> MKQGFARPTPERAPVVKPENIVLPTPLSVPPPEGKPWWLVVVGVLVVGLLVGMVGMTVASGSRLFLGAGAIFPIFMIGGVAMMMFGGRFGGQQQMSRPKLDAMRAQFMLMLDMLRETAQESADSMDANYRWFHPAPTTLAAAVGSSRMWERQPDGKDLNFGVVRVGVGMTRPEVTWGEPQNMPTDIELEPVTGKALQEFGRYQSVVYNLPKMVSLLVEPWYSLVGEREQVLGLTRAIICQLAFSHGPDHVQMIVVTSDPDRWDWVKWIPHFGDPRRRDAAGNARMVYTSVREFATEQAELFAGRGSFTPRHASSSAETPTPHHVIISDIEDPQWEYVISSEGVDGVTFFDLTGSPLWTGAPQRVLRFTDSAGVIETLPRDRDTWMVIDDNAWFFALADQMSEADAEQFAHQMAHWRLAEAYEEIGQRVVQLGARDILSYYGIDDAGEIDFNT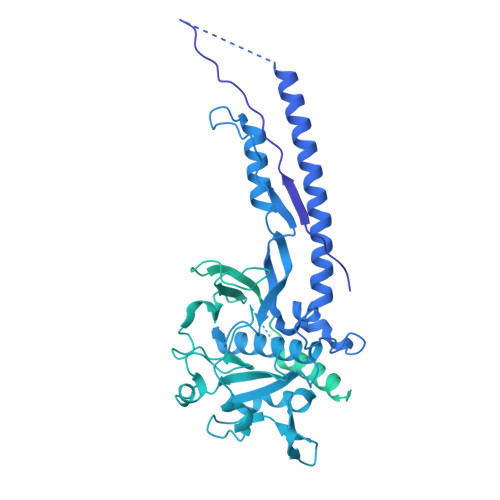LWSGSGRRDLLSRSRLRIPFGNRADNGELLFLDMKSLDEGGDGPHGVMSGTTGSGKSSLVRTVIASLMLAHPPEELQFVLADLKGGSAVKPFDGVPHVSRIITDLEDDQALMERFLEAMWGEIARRKEICFSAGVDGAKEYNELRARMKARGEDMPPLPMLVVVIDEFYEWFRIMPTAVDVLDSIGRQGRAYWVHLMMASQTIESRAEKLMENMGYRLVLKAQTAGAAQAAGVPNAVNLPSQAGLGYFRKSGDEIIRFQAEYLWRDYRRGSSYDGEEQAPLTHSVDYIRPQLFTTAFAPLEVSVSGPDGQSALPQVVDGEAVNGHRGGDDVDEEEEALRTPKVGTVIIDQLRQIDFEPYRLWHPPLDVPVPIDELVNRFLGRPWQQDYGTAKNLVFPIGIIDRPYKHDQPPWTVDTSGAGANVLILGAGGAGKTTALQTLICAAALTHTPEQVQFYCLAYSGTALTTVANLPHVGGVSGPTDPYGVRRTVAEVLGLVRDRKRSFLEYDVPSMEVFRRRKFGGEPGGVPDDGFGDVYLVIDNYRALAEENEVLIEQVNQIINQGPSFGVHVVATADRESELRPPVRSGFGSRVELRLAAVEDAKLVRSRFAKDVPPKPGRGMVAVNYVRLDSDPQAGLHTLVARPALGSTPDAVFESDSVAAAVRQVAAGEARPVRRLPARFGLDQLRQVAAADRRQGVGAGGIAWAISELDLQPVYLNFADNAHLMVTGRRECGRTTTLATIMSEIGRIYAPGASTAPPTSRPSAQVWLVDPRRQLLTVLGSDYVEKFAYNLDGVAAMMDDLAAALARREPPPGLSAEELLSRSWWSGPEIFLIIDDIQQLPPGFDSPLHKAAPWVTRAADVGLHVFVTRTFGGWSSAGSDPILRALHQANAPLLVMDADPDEGFIRGKMKGGPLPRGRGLLMAEDTGVFVQVAATDLRR> IINGEDCSPHSQPWQAALVMENELFCSGVLVHPQWVLSAAHCFQNSYTIGLGLHSLEADQEPGSQMVEASLSVRHPEYNRPLLAND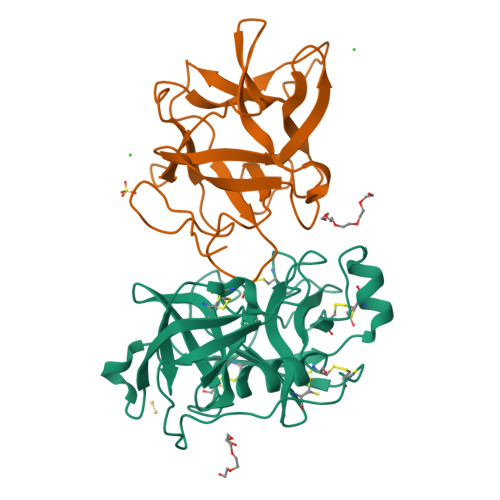LMLIKLDESVSESDTIRSISIASQCPTAGNSCLVSGWGLLANGRMPTVLQCVNVSVVSEEVCSKLYDPLYHPSMFCAGGGQDQKDSCNGDSGGPLICNGYLQGLVSFGKAPCGQVGVPGVYTNLCKFTEWIEKTVQA;> GSSVVVDTNGQPVSNGADAYYLVPVSHGHAGLALAKIGNEAEPRAVVLDPHHRPGLPVRFESPLRINIIKESYFLNIKFGPSSSDSGVWDVIQQDPIGLAVKVTDTKSLLGPFKVEKEGEGYKIVYYPERGQTGLDIGLVHRNDKYYLAVKDGEPCVFKIRKATDE>[2x]AHMFERVKTFQVPSPSIGTLPPAPDFKNDINEQLPDKTNPVITHFSTIPYIMANDATFNSHQQIQYSPYYKLVRIQYWEKVTQRILGPR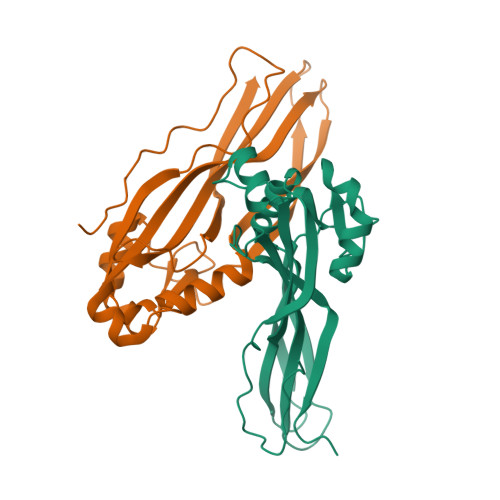DDYEYNKTKGISKTDQVSMTETVSMSVGADFGFMFKGFSASLSAQITKELSVTKSTSTTEMTEETYKEKYTNPFNYELARAQYMLVNEFYVTRMDGTRITANWTLRDNTQTVTRIFPKS> GAEFKGLRRHMFLYNLTLQRATGISFAIHGNFSGTKQQEIVVSRGKILELLRPDPNTGKVHTLLTVEVFGVIRSLMAFRLTGGTKDYIVVGSDSGRIVILEYQPSKNMFEKIHQETFGKSGCRRIVPGQFLAVDPKGRAVMISAIEKQKLVYILNRDAAARLTISSPLEAHKANTLVYHVVGVDVGFENPMFACLEMDYEEADNDPTGEAAANTQQTLTFYELDLGLNHVVRKYSEPLEEHGNFLITVPGGSDGPSGVLICSENYITYKNFGDQPDIRCPIPRRRNDLDDPERGMIFVCSATHKTKSMFFFLAQTEQGDIFKITLETDEDMVTEIRLKYFDTVPVAAAMCVLKTGFLFVASEFGNHYLYQIAHLGDDDEEPEFSSAMPLEEGDTFFFQPRPLKNLVLVDELDSLSPILFCQIADLANEDTPQLYVACGRGPRSSLRVLRHGLGGNGNSGEKLGAVFNQVAFPLQYTPRKFVIH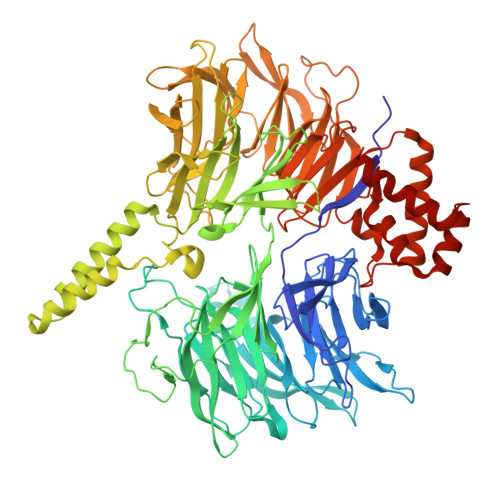PESNNLIIIETDHNAYTEATKAQRKQQMAEEMVEAAGEDERELAAEMAAAFLNENLPESIFGAPKAGNGQWASVIRVMNPIQGNTLDLVQLEQNEAAFSVAVCRFSNTGEDWYVLVGVAKDLILNPRSVAGGFVYTYKLVNNGEKLEFLHKTPVEEVPAAIAPFQGRVLIGVGKLLRVYDLGKKKLLRKCENKHIANYISGIQTIGHRVIVSDVQESFIWVRYKRNENQLIIFADDTYPRWVTTASLLDYDTVAGADKFGNICVVRLPPNTNDEVDSQKAEVIMNYHVGETVLSLQKTTLIPGGSESLVYTTLSGGIGILVPFTSHEDHDFFQHVEMHLRSEHPPLCGRDHLSFRSYYFPVKNVIDGDLCEQFNSMEPNKQKNVSEELDRTPPEVSKKLEDIRTRYAQLEQNEAAF Prenyltransferases, also known as isoprenyl diphosphate synthases, catalyze the sequential condensation of a basic five-carbon building block (C5), the isopentenyl diphosphate (IPP), to synthesize prenyl precursors of isoprenoid metabolites and isoprene polymers, collectively called polyisoprene. Ultrahigh molecular weight cis-1,4-polyisoprene and trans-1,4-polyisoprene (TPI), which are the principal components of natural rubber and gutta-percha, respectively, are also isoprenoid metabolites that are assumed to be synthesized by specialized prenyltransferases. These prenyltransferases are divided into two major groups, the cis-1,4-prenyltransferases (CPTs) and trans-1,4-prenyltransferases (TPTs), based on the stereochemistry of the double bond formed during IPP condensation. To investigate the molecular properties of the EuTPT proteins, we determined the three-dimensional structures of EuTPT3 and EuFPS1 using X-ray crystallography. Similar to EuFPS1 and other prenyltransferases, the EuTPT3 subunits were composed of 10 core helices (α1-α10) with a deep pocket that included two DDxxD motifs responsible for substrates binding.

The crystal structure of apo EuTPT3 was determined from two crystal forms with space groups P43212 and C2, refined at 3.0 and 3.3 Å resolution, respectively. All dimers observed in the two crystal forms were superimposable with a root-mean-square deviation (RMSD) range of 0.797–0.941 Å over 595–633 aligned Cα atoms. The superimposition parameters suggested that the dimeric architecture of EuTPS3 was highly conserved and unlikely to be caused by crystal packing. In EuTPT3, α6 of one subunit interacted with α5 and α6 of the neighboring subunit to form a four-helix bundle, whereas, in EuFPS1, α4 of one subunit was inserted between α5 and α6 of the neighboring subunit to form a six-helix bundle of α4–α6 at the dimer interface. Thus, EuTPT3 had a larger central tunnel than EuFPS1. Our structural analysis identified a unique, TPT-type dimer conformation, in which the central tunnel connected the active site with the bottom of the molecule. Crystal structure of EuTPT3 showed that the residues Ile164-Ala165 contact with Ile164 and Ile125 of the neighboring subunit in the hydrophobic tunnel, suggesting that smaller side chains such as valine and glycine provide the wider path for the product that may contribute to the activity difference. Furthermore, EuTPT3 conserved a hydrophobic hollow in the bottom region of the dimer interface. These observations suggested that the longer polyisoprene products may pass through the hydrophobic tunnel at the dimer interface.

>[7x]MNHKVHHHHHHIEGRHMTELKSKFVKVYSVLKKELLHDSAFGLTDDSRNWVERIMDYNVPGGKLNRGLSVVDSYKLLRELTNSKYKSELSDDEIFLASVLGWSVEWIQACALVLDDIMDHSHTRRGHPCWFRLPKVGMIAINDGLILRNHVPRILRTHFQTEHYYLQLVDLFHEVECQTIAGQMLDLITTLAGEINLSSYSLPVYQQITLSKTSYYSFYLPVACALVMLGENLESHDDMKDILLEMGTYFQVQDDYLDCFGDPEVIGKIGTDIEDNKCTWLVVQALEHCNEEQKKLLYDNYGRKDPKQVAKVKELYKTLNLEDLFTQYENKTCKKLTKSIEALPNVAVQAVLKSFLAKIHKRLK> MSMLVVVTENVPPRLRGRLAIWLLEVRAGVYVGDVSAKIREMIWEQIAGLAEEGNVVMAWATNTETGFEFQTFGLNR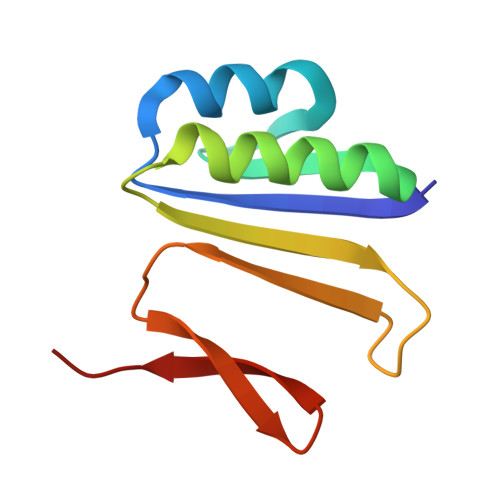RTPVDLDGLRLVSFLPV Death-associated protein kinase (DAPK) is a member of the Ca2+/calmodulin-regulated family of serine/threonine protein kinases. The role of the kinase activity of DAPK in eukaryotic cell apoptosis and the ability of bioavailable DAPK inhibitors to rescue neuronal death after brain injury have made it a drug-discovery target for neurodegenerative disorders. The three DAPK conformations demonstrate that nucleotide binding brings about changes in conformation that are mostly localized to the glycine-rich loop region. The most notable conformational changes occur in the glycine-rich loop region, an active-site region with potential for modulation of kinase activity.

In this alternative conformation, the phosphate is in a similar location to the position where Mg2+ binds. This raises the possibility that the role of Mg2+ is to assist in the selection of a catalytically preferred conformation of the β-­phosphate.

> TVFRQENVDDYYDTGEELGSGQFAVVKKCREKSTGLQYAAKFIKKRRTKSSRRGVSREDIEREVSILKEIQHPNVITLHEVYENKTDVILILELVAGGELFDFLAEKESLTEEEATEFLKQILNGVYYLHSLQIAHFDLKPENIMLLDRNVPKPRIKIIDFGLAHKIDFGNEFKNIFGTPEFVAPEIVNYEPLGLEADMWSIGVITYILLSGASPFLGDTKQETLANVSAVNYEFEDEYFSNTSALAKDFIRRLLVKDPKKRMTIQDSLQHPWIKPKDTQQALSSAWSHPQFEK> GSRKTCRYIPSLPDRILDAPEIRNDYYLNLVDWSSGNVLAVALDNSVYLWSASSGDILQLLQMEQPGEYISSVAWIKEGNYLAVGTSSAEVQLWDVQQQKRLRNMTSHSARVGSLSWNSYILSSGSRSGHIHHHDVRVAEHHV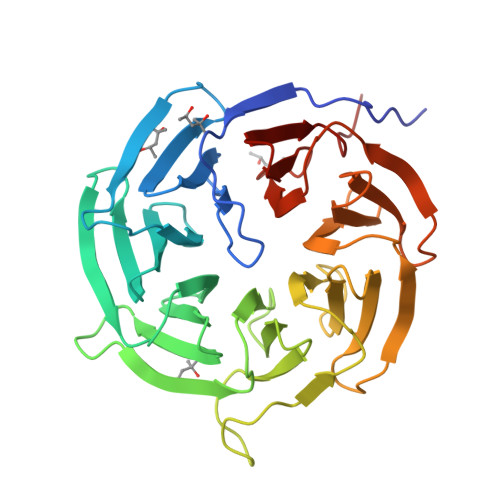ATLSGHSQEVCGLRWAPDGRHLASGGNDNLVNVWPSAPGEGGWVPLQTFTQHQGAVKAVAWCPWQSNVLATGGGTSDRHIRIWNVCSGACLSAVDAHSQVCSILWSPHYKELISGHGFAQNQLVIWKYPTMAKVAELKGHTSRVLSLTMSPDGATVASAAADETLRLWRCFELDP Using a combination of biochemical and crystallographic methods we show that E. coli TldD and TldE interact to form a heterodimeric metalloprotease. TldD/E cleaves the N-terminal leader sequence from the modified MccB17 precursor peptide, to yield mature antibiotic, while it has no effect on the unmodified peptide. Both proteins are essential for the activity; however, only the TldD subunit forms a novel metal-containing active site within the hollow core of the heterodimer. Peptide substrates are bound in a sequence-independent manner through β sheet interactions with TldD and are likely cleaved via a thermolysin-type mechanism.

The structure of the purified TldD/E protein complex was solved from a 1.9-Å resolution dataset (WT-PO4) using molecular replacement with templates based on structures that were 23% and 99% identical in sequence to TldD and TldE, respectively, to give two copies of the TldD/E heterodimer in the asymmetric unit. These are roughly spherical, resembling the previously crystallized TldE (PmbA) homodimers, with an average outer diameter of approximately 65 Å and a hollow core. In the TldD/E structure, the TldD HExxxH motif, spanning residues 262–267, is located on the central helix that resides within the β funnel, and with the two histidine residues, His262 and His267, coordinating a metal ion, which we modeled as Zn (because Zn was added to the growth medium); a third ligand is provided by Cys454 from the clamp domain. In our first determined structure of TldD/E, a phosphate anion (derived from the crystallization solution, hence WT-PO4) serves as a fourth ligand to the zinc, which is also held by a bidentate interaction with Glu263. An oxygen atom of this bound phosphate corresponds to the position of the “catalytic” water molecule in thermolysin. The resultant negatively charged tetrahedral intermediate is stabilized through interactions with the zinc; this stage of the reaction is mimicked by the phosphate-bound TldD/E structure. In the absence of adventitiously bound ligands, we expect the fourth zinc coordination site of TldD to be occupied by a water molecule.

>MGSSHHHHHHSQDPMSLNLVSEQLLAANGLKHQDLFAILGQLAERRLDYGDLYFQSSYHESWVLEDRIIKDGSYNIDQGVGVRAISGEKTGFAYADQISLLALEQSAQAARTIVRDSGDGKVQTLGAVEHSPLYTSVDPLQSMSREEKLDILRRVDKVAREADKRVQEVTASLSGVYELILVAATDGTLAADVRPLVRLSVSVLVEEDGKRERGASGGGGRFGYEFFLADLDGEVRADAWAKEAVRMALVNLSAVAAPAGTMPVVLGAGWPGVLLHEAVGHGLEGDFNRRGTSVFSGQVGELVASELCTVVDDGTMVDRRGSVAIDDEGTPGQYNVLIENGILKGYMQDKLNARLMGMTPTGNGRRESYAHLPMPRMTNTYMLPGKSTPQEIIESVEYGIYAPNFGGGQVDITSDKFVFSTSEAYLIENGKVTKPVKGATLIGSGIETMQQISMVGNDLKLDNGVGVCGKEGQSLPVGVGQPTLKVDNLTVGGTA[2x];>MALAMKVISQVEAQRKILEEAVSTALELASGKSDGAEVAVSKTTGISVSTRYGEVENVEFNSDGALGITVYHQNRKGSASSTDLSPQAIARTVQAALDIARYTSPDPCAGVADKELLAFDAPDLDLFHPAEVSPDEAIELAARAEQAALQADKRITNTEGGSFNSHYGVKVFGNSHGMLQGYCSTRHSLSSCVIAEENGDMERDYAYTIGRAMSDLQTPEWVGADCARRTLSRLSPRKLSTMKAPVIFANEVATGLFGHLVGAIAGGSVYRKSTFLLDSLGKQILPDWLTIEEHPHLLKGLASTPFDSEGVRTERRDIIKDGILTQWLLTSYSARKLGLKSTGHAGGIHNWRIAGQGLSFEQMLKEMGTGLVVTELMGQGVSAITGDYSRGAAGFWVENGEIQYPVSEITIAGNLKDMWRNIVTVGNDIETRSNIQCGSVLLPEMKIAGQ[2x]>[4x]HSTEEGLFSQKSFLVLGFSNENESNIANIIKENAGKIMSLLSRTVADYAVVPLLGCEVEATVGEVVTNTWLVTCIDYQTLFDPKSNPLFTPVPVMTGMTPLEDCVISFSQCA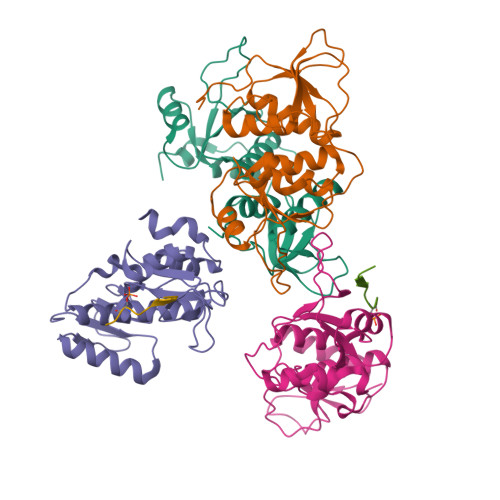GAEKESLTFLANLLGASVQEYFVRKSNAKKGMFASTHLILKERGGSKYEAAKKWNLPAVTIAWLLETARTGKRADESHFLIENS;>SSDLVAPSPDAFRST[2x]>SKHGLTKEMTMKYRMEGCVDGHKFVITGEGIGYPFKGKQAINLCVVEGGPLPFAEDILSAAFDYGNRVFTEYPQDIVDYFKNSCPAGYTWDRSFLFEDGAVCICNADITVSVEENCMYHESKFYGVNFPADGPVMKKMTDNWE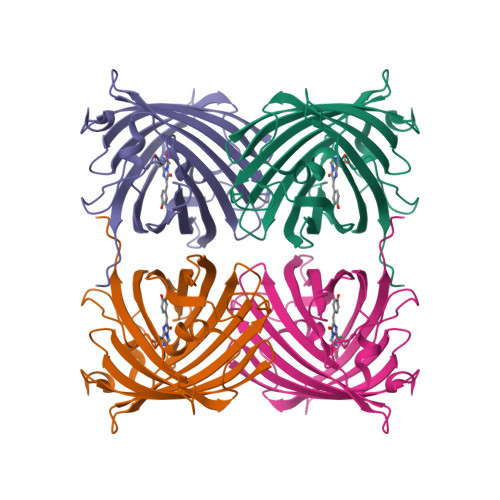PSCEKIIPVPKQGILKGDVSMYLLLKDGGRLRCQFDTVYKAKSVPRKMPDWHFIQHKLTREDRSDAKNQKWHLTEHAIASGSALP[2x]>GKKKVCYYYDGDIGNYYYGQGHPMKPHRIRMTHNLLLNYGLYRKMEIYRPHKATAEEMTKYHSDEYIKFLRSIRPDNMSEYSKQMQRFNVGEDCPVFDGLFEFCQLSTGGSVAGAVKLNRQQTDMAVNWAGGLHHAKKSEASGFCYVNDIVLAILELLKYHQRVLYIDIDIHHGDGVEE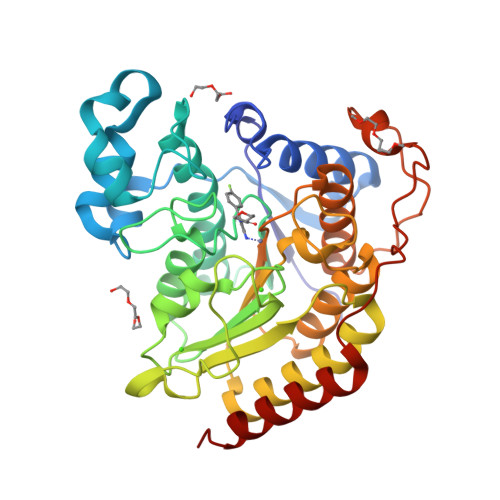AFYTTDRVMTVSFHKYGEYFPGTGDLRDIGAGKGKYYAVNFPMRDGIDDESYGQIFKPIISKVMEMYQPSAVVLQCGADSLSGDRLGCFNLTVKGHAKCVEVVKTFNLPLLMLGGGGYTIRNVARCWTYETAVALDCEIPNELPYNDYFEYFGPDFKLHISPSNMTNQNTPEYMEKIKQRLFENLRMLP[3x]> MAIYEINGKKPRIHPSAFVDENAVVIGDVVLEEKTSVWPSAVLRGDIEQIYVGK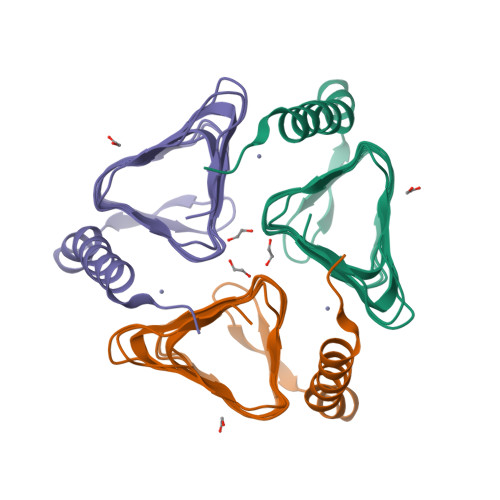YSNVQDNVSIHTSHGYPTEIGEYVTIGHNAMVHGAKVGNYVIIGISSVILDGAKIGDHVIIGAGAVVPPNKEIPDYSLVLGVPGKVVRQLTEEEIEWTKKNAEIYVELAEKHIKGRKRI>[33x]MAQVINTNSLSLITQNNINKNQSALSSSIERLSSGLRINSAKDDAAGQAIANRFTSNIKGLTQAARNANDGISVAQTTEGALSEINNNLQRIRELTVQASTGTNSDSDLDSIQDEIKSRLDEIDRVSGQTQFNGVNVLAKDGSMKIQVGANDGQTITIDLKKIDSDTLGLNGFNVNGKGETANTAATLKDMSGFTAAAAPGGTVGVTQYTDKSAVASSVDILNAVAGADGNKVTTSADVGFGTPAAAVTYTYNKDTNSYSAASDDISSANLAAF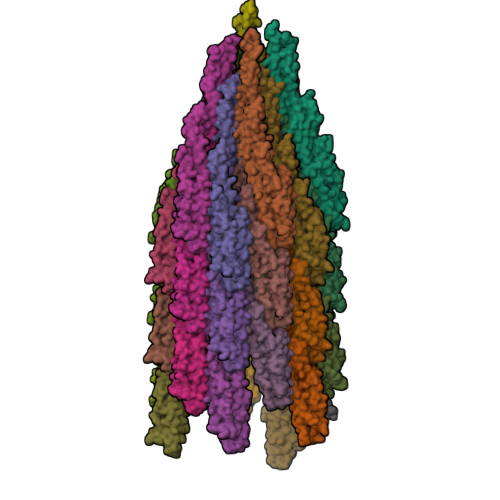LNPQARDTTKATVTIGGKDQDVNIDKSGNLTAADDGAVLYMDATGNLTKNNAGGDTQATLAKVATATGAKAATIQTDKGTFTSDGTAFDGASMSIDANTFANAVKNDTYTATVGAKTYSVTTGSAAADTAYMSNGVLSDTPPTYYAQADGSITTTEDAAAGKLVYKGSDGKLTTDTTSKAESTSDPLAALDDAISQIDKFRSSLGAVQNRLDSAVTNLNNTTTNLSEAQSRIQDADYATEVSNMSKAQIIQQAGNSVLAKANQVPQQVLSLLQG>MGSITENTSWNKEFSAEAVNGVFVLCKSSSKSCATNDLARASKEYLPASTFKIPNAIIGLETGVIKNEHQVFKWDGKPRAMKQWERDLTLRGAIQVSAVPVFQQIAREVGEVRMQKYLKKFSYGNQNISGGIDKFWLEGQLRISAVNQVEFLESLYLNKLSASKENQLIVKEALVTEAAPEYLVHSKTGFSGVGTESNPGVAWWVGWVEKETEVYFFAFNMDIDNESKLPLRKSIPTKIMESEGIIGG[2x]

The β-lactamase-catalysed hydrolysis of β-lactam antibiotics (BLAs) is of central importance in antibiotic resistance1. β-Lactam-based inhibitors (for example clavulanic acid) of the Class A serine-β-lactamases (SBLs) are widely used in combination with penicillins. We demonstrate through biochemical, biophysical and cellular evidence that cyclic boronates are potent inhibitors of both SBLs and MBLs. The cyclic boronates act as ‘transition state analogues' for both ‘serine' and ‘metallo' enzymes and therefore represent a promising strategy for combating antibiotic resistance. The combined results reveal that cyclic boronates act as dual action inhibitors of SBLs and MBLs by mimicking a common high-energy tetrahedral intermediate; they also reveal that cyclic boronates can potently inhibit some PBPs via the same mechanism.

We then investigated the binding mode of the cyclic boronates to SBLs, by determining a high-resolution crystal structure of the Class D β-lactamase OXA-10 in complex with 1 (1.5 Å resolution). OXA-10 requires a carbamylated active site lysine (KCX70) for catalysis, which was observed in the OXA-10:1 complex structure. Inspection of maps reveals continuous electron density connecting the inhibitor boron atom with the terminal hydroxyl group of the nucleophilic serine (Ser67) and provides clear evidence for a tetrahedral boron atom, contrasting with the planar geometry of the carbonyl carbon atoms of β-lactam acyl-enzyme complexes. The structure of the complex with 1 thus represents a covalent species that better resembles the ‘first' tetrahedral intermediate, which is involved in acyl-enzyme formation, rather than the acyl-enzyme itself. Hence, analogous to our structural observations with the VIM-2 and BcII MBLs (above), the OXA-10:1 complex structure reveals that 1 mimics the mechanistically important tetrahedral oxyanion that is transiently present on the hydrolytic pathway. Furthermore, comparison of the OXA-10:1 complex with that of a penicillin (benzylpenicillin) bound to a ‘deacylation-deficient' OXA-10 (K70C variant)23 reveals strikingly related overall binding modes. In particular, the carboxylate of 1 and the C-3 carboxylate of penicillin are both positioned to interact with Arg250, while the acetamido group of 1 and the benzylpenicillin C6 amide group are analogously positioned to hydrogen bond with the main chain carbonyl of Phe208. Finally, the endocyclic boronate ester oxygen of 1 and the β-lactam-derived nitrogen (from the penicillin thiazolidine ring) are both positioned to hydrogen bond with Ser115. All of the compounds tested were potent TEM-1 inhibitors (IC50 6→0.3 nM) and compounds with saturated side chains (1 and 3) manifested IC50 values<1 μM against OXA-10.>[2x]GMRQPFQVLVIPFIKTEANYQFGVLHRTDADVWQFVAGGGEDEEAI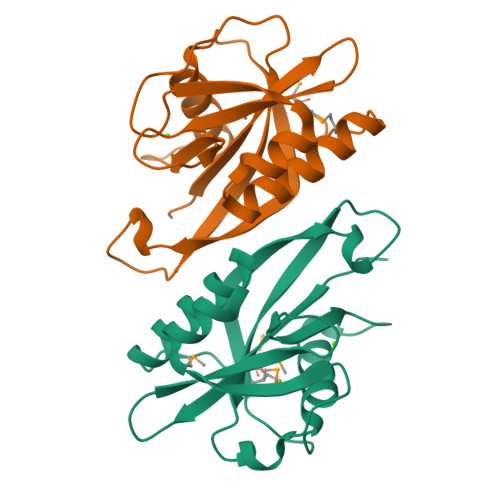SETAKRESIEELNLDVDVKMYSLDSHASIPNFHFSFNKPYVVPEYCFAIDLTSCSYQVTLSLEHSELRWVSYESAIQLLEWDSNKTALYELNERLKNNDMKAM>SKPFTVPILTVEEMTNSRFPIPLEKLFTGPSGAFVVQPQNGRCTTDGVLLGTTQLSPVNICTFRGDVTHIAGSRNYTMNLASLNWNNYDPTEEIPAPLGTPDFVGKIQGLLTQTTKGDGSTRGHKATVYTGSAPFTPKLGSVQFSTDTENDFETHQNTKFTPVGVIQDGSTTHRNEPQQWVLPSYSGRNVHNVHLAPAVAPTFPGEQLLFFRSTMPGCSGYPNMDLDCLLPQEWVQHFYQEAAPAQSDVALLRFVNPDTGRVLFECKLHKSGYV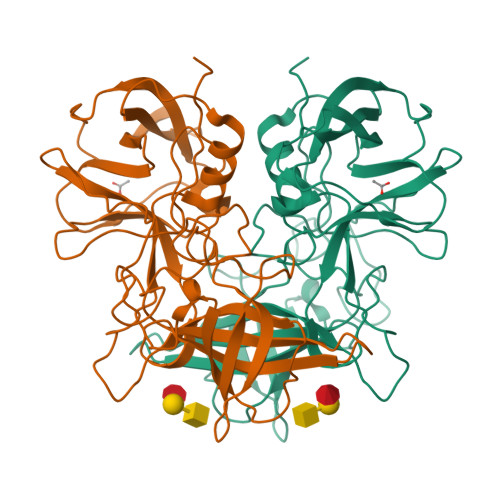TVAHTGQHDLVIPPNGYFRFDSWVNQFYTLAPM[2x]>[4x]AFYKREMFDPAEKYKMDHRRRGIALIFNHERFFWHLTLPERRGTCADRDNLTRRFSDLGFEVKCFNDLKAEELLLKIHEVSTVSHADADCFVCVFLSHGEGNHIYAYDAKIEIQT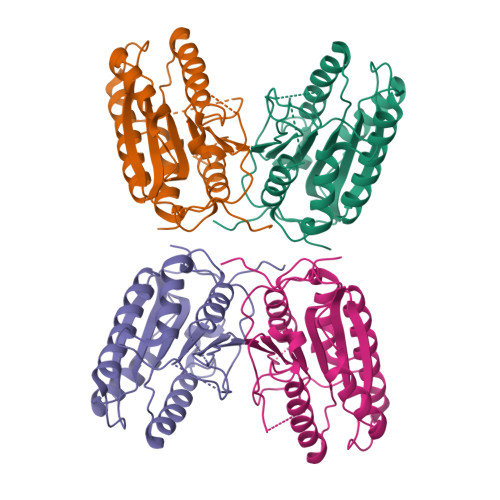LTGLFKGDKCHSLVGKPKIFIIQACRGNQHDVPVIPLDVVDNQTEKLDTNITEVDAASVYTLPAGADFLMCYSVAEGYYSHRETVNGSWYIQDLCEMLGKYGSSLEFTELLTLVNRKVSQRRVDFCKDPSAIGKKQVPCFASMLTKKLHFFPKSNLEHHHHHH4-(6-{[(4-METHYLCYCLOHEXYL)AMINO]METHYL}-1,4-DIHYDROINDENO[1,2-C]PYRAZOL-3-YL)BENZOIC 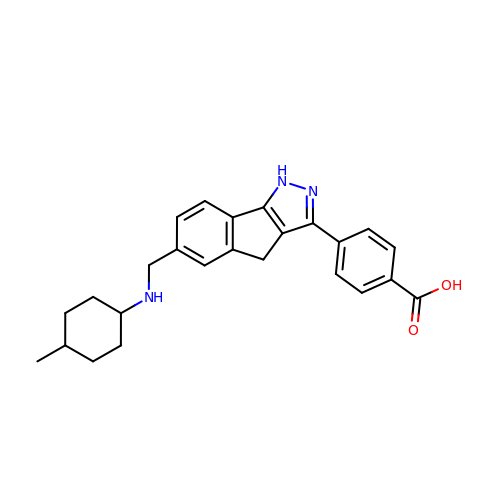ACID | C25 H27 N3 O2 | MEDLHZCDTXWLOC-GSXCWMCISA-N> MIMEIPAIKALSRYAQWVIWKKAADTKIPYNPNNGKKASSTDPLAWGDIDEAQAGLVRYGANGLGFVLTKSDPFVFIDLDHV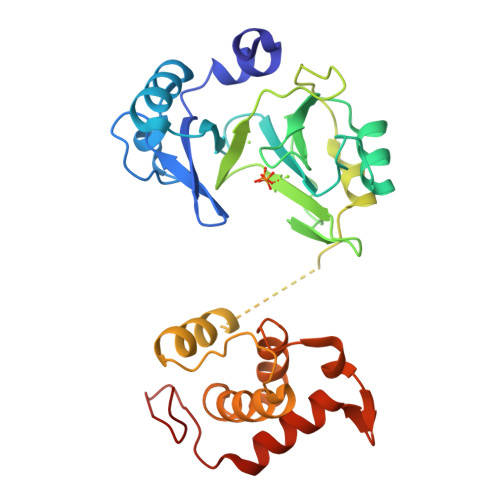LDENKRVKCEWARQLLKEIKSYTEISPSGDGLHVVVSGKLPDYIKHKTKFDDGSALEVYESGRYMTITGEVFDGRDDIKELDLSILGEFAEHKIETKNAPVQIESATTLDDEAIIDLMKRKGQWPDAPADGDDWSSLDMSFANRLAFWCGKDIERMDRIFRQSPLMRQKWDRPTAGSTYGRITLKKACDFVDSVYDPALRNESDCP>[2x]MENLGDKLSISQVYHLAQEYRDHAYSIANKIGSEEGLKQYYGLMNMSIQMFQLLKTKCTLSVLEDSKVTFEMVELLIQETYNFDLAELYISSLKERLQTHQSDTDLVEEIMRCEFLLLHDLPLMRDSKFHYKIALRNCNELVQYMVNLQDELYQNWASVFQYVGVM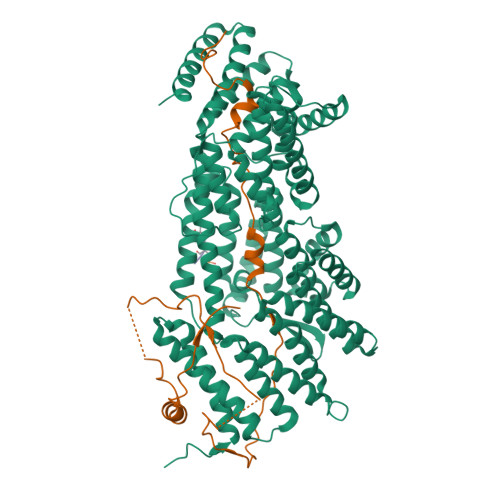LCIKLKQHRRVKTSFHGLLSQCREKSQWKWFLNLCYVNYLLNERFPIPEDALQELRSTELHTVGPELYAWKLALEMVIQLCKDGNITDHLNEFKNFFDTNKQSLVTNEGKGCVIKIMPRIALKVELPMIFHYKELKNILLLLQSVSYIVNCYDEKGNFSRKFLPKVYSTTQKLIKNIAAGGVSMNELDSRIQTYKSILEFCEFYKVWEQTLLKGAVVTTESPKLGPSPGYVRLLQAMKVQFEGGGAVEEYTRLAQSGGTSSEVKMISLLNCYTVQAARVSRCSGDKQGELVEQCNKVWLQVEKLLQETDLQFNPIWECTVTILWLFSHFEPFSWNPLPCSDKQRAEYVSKLREFYSSNKFVAGEAVADNRFKLKKALLLQILVNYLGGRMLEHDLGEIYAISAKCFDMCRQQGGMRKVQYVIGIWHLMNCTVAMRGKDVALTNAKLEALVKQITSVKQ;>SNAMSYPGKDKNIPGRIIEALEDLPLSYLVPKDGLAALVNAPMRVSLPFDKTIFTSADDGRDVNINVLGTANSTTSSIKNEAEKERLVFKRPSNFTSSANSVDYVPTNFLEGLSPLAQSVLSTHKGLNDSINIEKKSEIVSRPEAKHKLESVTSNAGNLSFNDNSSNKKTKTSTGVTMTQANLA[2x];>[2x]MDFTSD> EDPVTGPEEVSGQEQGSLTVQCRYTSGWKDYKKYWCQGVPQRSCKTLVETDASEQLVKKNRVSIRDNQRDFIFTVT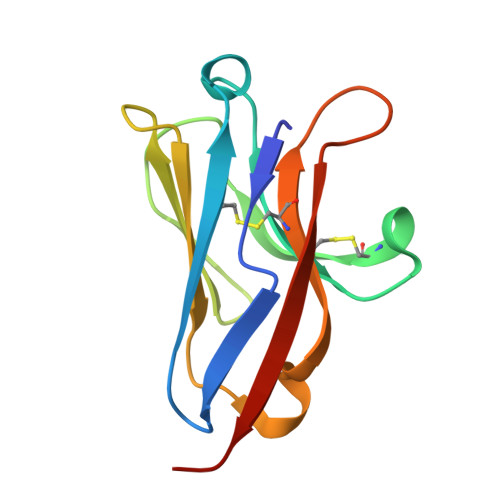MEDLRMSDAGIYWCGITKGGLDPMFKVTVNIGPVPT>[2x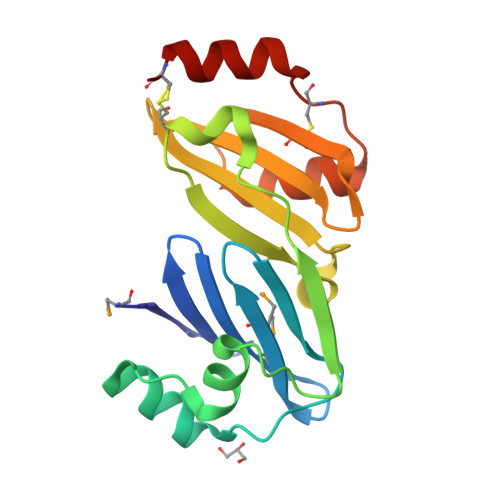]MYSVKKSKSGYIFDKPRERIAFMFLKDGTYFMYHDGRILCYSLKPVDVSREELEEFERTGEPPELIKRVKAGKYPENCVVKELPPIDKGLAQLNPNRKCVIIFTGFQDTVIDYVECNGETLAVARLIDEPGKVCRFAGKGNYKVAAVKLKRNEPCLTREEFLKKVEECRK Ornithine decarboxylase (ODC) is a pyridoxal phosphate (PLP)-dependent enzyme that catalyzes the conversion of ornithine to putrescine, a rate-limiting first step for the tightly regulated biosynthesis of polyamines (putrescine, spermidine, spermine).1−3 At the molecular level, positively charged polyamines interact with negatively charged RNA, DNA, and phospholipids, thereby directly contributing to chromatin biology. The ODC enzyme is a homodimer, with the dimer interface forming its catalytic site from residues from both monomers. We report two X-ray structures of ODC complexed with new ODC inhibitors, computational docking, molecular dynamics, and binding free energy calculations to validate the experimental models. The X-ray structures reveal that covalent adducts with pyridoxal phosphate (PLP) are formed in the active site of the human ODC enzyme, as verified by their preparation and enzymatic testing.

We then turned our attention to the inclusion of the 5-membered pyrrolidine analogs. Compounds 10, 10-R and 10-S had ODC IC50 values of 0.36, 0.21, and 0.10 μM, respectively. Like that observed for the piperidine derivatives (7-R and -S), the IC50s values are only slightly differentiated favoring the S-enantiomer and in a range similar to that observed for APA. As before, it is anticipated that the PLP adducts are formed in the active site and are the true inhibitors. To help verify, we have also prepared 10-R-PLP and 10-S-PLP and found that they both demonstrate inhibition of ODC enzymatic activity, with IC50 values of 0.16 and 0.03 μM, respectively. The activity still favors, as observed for 10-R and -S, the S-enantiomer with 8-fold relative activity. In each case, as we saw with APA, the adducts 10-R-PLP (2.9 Å resolution) and 10-S-PLP (2.0 Å resolution) were formed, forming trans-oximes with PLP. The lipophilic cyclic pyrrolidines of 10-R-PLP and -S-PLP, form strong lipophilic interactions with Tyr389 and weaker lipophilic interactions with Phe397, the pyrrolidine rings orientated in an orthogonal manner relative to each other. The basic pyrrolidine amine of each makes a H-bonding interaction with Asp331.

>[2x]MNNFGNEEFDCHFLDEGFTAKDILDQKINEVSSSDDKDAFYVADLGDILKKHLRWLKALPRVTPFYAVKCNDSKAIVKTLAATGTGFDCASKTEIQLVQSLGVPPERIIYANPCKQVSQIKYAANNGVQMMTFDSEVELMKVARAHPKAKLVLRIATDDSKAVCRLSVKFGATLRTSRLLLERAKELNIDVVGVSFHVGSGCTDPETFVQAISDARCVFDMGAEVGFSMYLLDIGGGFPGSEDVKLKFEEITGVINPALDKYFPSDSGVRIIAEPGRYYVASAFTLAVNIIAKKIVLKEQTGSDDEDESSEQTFMYYVNDGVYGSFNCILYDHAHVKPLLQKRPKPDEKYYSSSIWGPTCDGLDRIVERCDLPEMHVGDWMLFENMGAYTVAAASTFNGFQRPTIYYVMSGPAWQLMQQFQNPD>[2x]NLIQFGNMIQCANKGSRPSLDYADYGCYCGWGGSGTPVDELDRC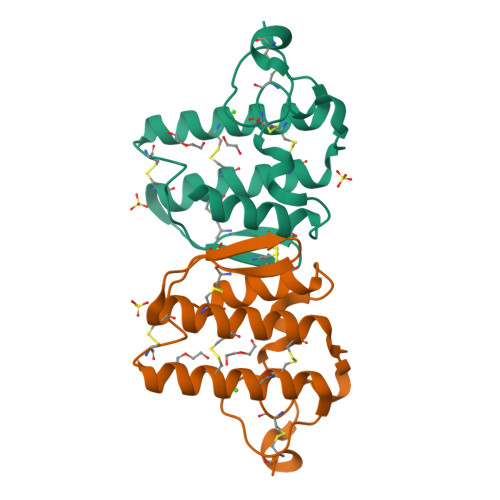CQVHDNCYEQAGKKGCFPKLTLYSWKCTGNVPTCNSKPGCKSFVCACDAAAAKCFAKAPYKKENYNIDTKKRCK>SNAPDNYFSGQQLTLARAIENGEVDEVIKLASGTDLNKPGKEDMTLLFWAVMNSINNQKTPERLNVITMLIKAGADPLQPRPQGKNSPAEFVLMADNADWIKAMLNAGLSPNAVDKTFGKPIIFQTLEAKNTKTLQAMLDKGADINITDSLGNTLLIDALDFHSYDHVLL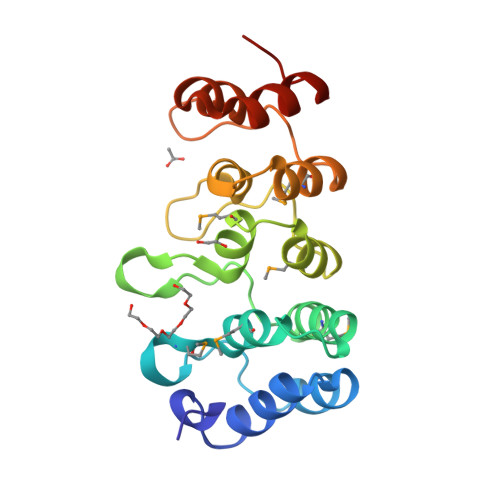LLERGADPEI[2x]>MGQVLPLVTRQGDRIAIVSGLRTPFARQATAFHGIPAVDLGKMVVGELLARSEIPAEVIEQLVFGQVVQMPEAPNIAREIVLGTGMNVHTDAYSVSRACATSFQAVANVAESLMAGTIRAGIAGGADSSSVLPIGVSKKLARVLVDVNKARTMSQRLKLFSRLRLRDLMPVPPAVAEYSTGLRMGDTAEQMAKTYGITREQQDALAHRSHQRAAQAWSDGKLKEEVMTAFIPPYKQPLVEDNNIRGNSSLADYAKLRPAFDRKHGTVTAANSTPLTDGAAAVILMTESRAKELGLVPLGYLRSYAFTAIDVWQDMLLGPAWSTPLALERAGLTMSDLTLIDMHEAFAAQTLANIQLLGSERFAREALGRAHATGEVDDSKFNVLGGSIAYGHPFAATGARMITQTLHELRRRGGGFGLVTACAAGGLGAAMVLEAE[2x];>MEMTSAFTLNVRLDNIAVITIDVPGEKMNTLKAEFASQVRAIIKQLRENKELRGVVFVSAKPDNFIAGADINMIGNCKTAQEAEALARQGQQLMAEIHALPIQVIAAIHGACLGGGLELALACHGRVCTDDPKTVLGLPEVQLGLLPGSGGTQRLPRLIGVSTALEMILTGKQLRAKQALKLGLVDDVVPHSILLEAAVELAKKERPSSRPLPVRERILAGPLGRALLFKMVGKKTEHKTQGNYPATERILEVVETGLAQGTSSGYDAEARAFGELAMTPQSQALRSIFFASTDVKKDPGSDAPPAPLNSVGILGGGLMGGGIAYVTACKAGIPVRIKDINPQGINHALKYSWDQLEGKVRRRHLKASERDKQLALISGTTDYRGFAHRDLIIEAVFENLELKQQMVAEVEQNCAAHTIFASNTSSLPIGDIAAHATRPEQVIGLHFFSPVEKMPLVEIIPHAGTSAQ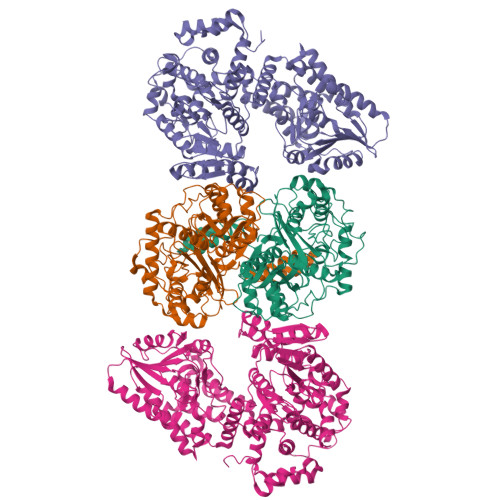TIATTVKLAKKQGKTPIVVRDKAGFYVNRILAPYINEAIRMLTQGERVEHIDAALVKFGFPVGPIQLLDEVGIDTGTKIIPVLEAAYGERFSAPANVVSSILNDDRKGRKNGRGFYLYGQKGRKSKKQVDPAIYPLIGTQGQGRISAPQVAERCVMLMLNEAVRCVDEQVIRSVRDGDIGAVFGIGFPPFLGGPFRYIDSLGAGEVVAIMQRLATQYGSRFTPCERLVEMGARGESFWKTTA[2x]Cytoplasmic polyhedrosis viruses (CPVs), like other members of the order Reovirales, produce viroplasms, hubs of viral assembly that shield them from host immunity. Our study investigates the potential role of NSP9, a nucleic acid-binding non-structural protein encoded by CPVs, in viroplasm biogenesis. NSP9 robustly binds to single- and double-stranded nucleic acids, regardless of RNA or DNA origin. The disordered C-terminal region of NSP9 facilitates oligomerization but is dispensable for nucleic acid binding.

Accordingly, we expressed a truncated NSP9 (NSP9ΔC, lacking residues 287–320) from BmCPV1 in E. coli as an N-terminally MBP-tagged protein. The purified NSP9ΔC existed as a dimer in solution, as confirmed by SEC and analytical ultracentrifugation (AUC), with a precise molar mass of 60.5 kDa. The purified NSP9ΔC was crystallized in an orthorhombic space group P212121, with unit cell dimensions of a = 82.4 Å, b = 83.6 Å and c = 184.4 Å. In the asymmetric unit, four molecules of NSP9ΔC were identified and organized into two virtually identical dimers, with a Root Mean Square Deviation (RMSD) of 0.6 Å. The final refined model achieved a high resolution of 1.80 Å, exhibiting favorable stereochemistry parameters and refinement statistics (Rwork = 0.18 and Rfree = 0.20). The overall structure of the NSP9ΔC subunit revealed a compact architecture composed of 8 α-helices (α1 to α8) and 13 β-strands (β1 to β13). The NSP9ΔC homodimer exhibits a distinctive awninged ship-like structure. The dimerization interaction of NSP9ΔC involves an interface area of approximately 1536 Å2 (11.5% of the total solvent-accessible surface per protomer) between protomers A and B, and approximately 1177 Å2 (9.6% of the total solvent-accessible surface per protomer) between protomers C and D due to the lack of the awning-like β-sheet II pairs, both larger than the homodimer interaction of MRCV P9-1 according to the PDBePISA server. The arch-shaped structure contains six positively charged amino acids, specifically R9, K10, K12, K20, K23 and R28, which span residues 8 to 28 and form the tunnel. The elucidated structure identified a positively charged tunnel surrounded by a compact NSP9ΔC dimer as the nucleic acid binding channel, thereby suggesting a plausible interaction potentially between the protein and the nucleic acid from both termini.

>AGFMEAFLLENRKPKITTLASGKTLKPATHRLNLPAYTKLIHELRTKTHAKVTISLSTESQIHMVWVKSGLVFFTPSASHPAYVNFASSSRLTDVPALTKPTFPQSDAKLIESTPLPNDEASHVASFQLVTWKDGALSILNDLSKCAISFINQCEDTFKSGTNLNKEMYNRCITAESRDFCNQMKFVLIGRLCYGQTTSPPPIQLYQYGVTPFISADIICEGAAYRSIDVENYAMNSNHLVSYAPFFVPNDTKPGSRIDLLMVNHLKKFNLIFDTWYKTGGSVMVSSRP[4x]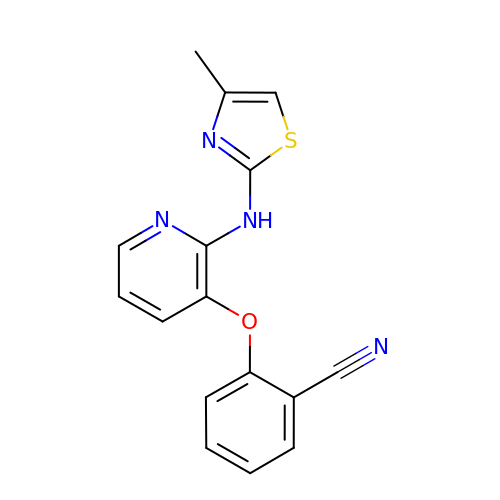2-({2-[(4-methyl-1,3-thiazol-2-yl)amino]pyridin-3-yl}oxy)benzonitrile | C16 H12 N4 O S | KPJJEXKLZAXHEE-UHFFFAOYSA-N> GPGGDPHMSKFTWKELIQLGSPSKAYESSLACIAHIDMNA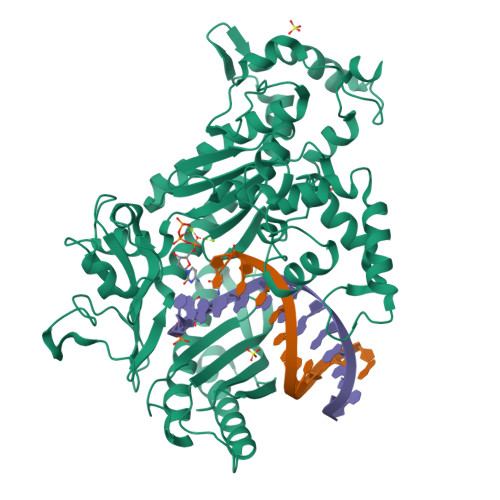FFAQVEQMRCGLSKEDPVVCVQWNSIIAVSYAARKYGISRMDTIQEALKKCSNLIPIHTAVFKKGEDFWQYHDGCGSWVQDPAKQISVEDHKVSLEPYRRESRKALAIFKWACDLVERASIDEVFLDLGRICFNMLMFDNEYELTGDLKLKDALSNIREAFIGGNYDINSHLPLIPEKIKSLKFEGDVFNPEGRDLITDWDDVILALGSQVCKGIRDSIKDILGYTTSCGLSSTKNVCKLASNYKKPDAQTIVKNDCLLDFLDCGKFEITSFWTLGGVLGKELIDVLDLPHENSIKHIRETWPDNAGQLKEFLDAKVKQSDYDRSTSNIDPLKTADLAEKLFKLSRGRYGLPLSSRPVVKSMMSNKNLRGKSCNSIVDCISWLEVFCAELTSRIQDLEQEYNKIVIPRTVSISLKTKSYEVYRKSGPVAYKGINFQSHELLKVGIKFVTDLDIKGKNKSYYPLTKLSMTITNFDIIDLQK>M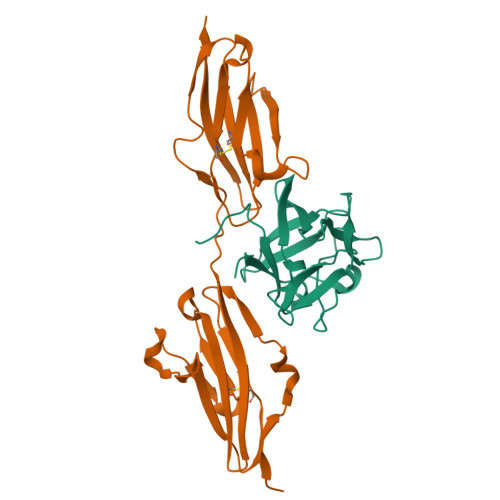AAGSITTLPALPEDGGSGAFPPGHFKDPKRLYCKNGGFFLRIHPDGRVDGVREKSDPHIKLQLQAEERGVVSIKGVSANRYLAMKEDGRLLASKSVTDECFFFERLESNNYNTYRSRKYTSWYVALKRTGQYKLGSKTGPGQKAILFLPMSAKS[4x];>[4x]NSNNKRAPYWTNTEKMEKRLHAVPAANTVKFRCPAGGNPMPTMRWLKNGKEFKQEHRIGGYKVRNQHWSLIMESVVPSDKGNYTCVVENEYGSINHTYHLDVVERSRHRPILQAGLPANASTVVGGDVEFVCKVYSDAQPHIQWIKHVEKNGSKYGPDGLPYLKVLKAAGVNTTDKEIEVLYIRNVTFEDAGEYTCLAGNSIGISFHSAWLTVLPAPGRE>[2x]GSHMMPQLQFKDAFWCRDFTAHTGYEVLLQRLLDGRKMCKDMEELLRQRAQAEERYGKELVQIARKAGGQTEINSLRASFDSLKQQMENVGSSHIQLALTLREELRSLEEFRERQKEQRKKYEAVMDRVQKSKLSLYKKAMESKKTYEQKCRDADDAEQAFERISANGHQKQVEKSQNKARQCKDSATEAERVYRQSIAQLEKVRAEWEQEHRTTCEAFQLQEFDRLTILRNALWVHSNQLSMQCVKDDELYEEVRLTLEGCSIDADIDSFIQAKSTGTEPPAPVPYQNYYD;> GFANRFSKPKGPRNPPPTWNI

PSTPIP1 is an adaptor protein expressed in most immune cell lineages. It presents two structural domains in its sequence, an N-terminal Fer/CIP4 homology-Bin/Amphiphysin/Rvs (F-BAR) domain and a C-terminal SH3 domain, connected by a linker region. The F-BAR domain of PSTPIP1 binds to the PEST subfamily of protein tyrosine phosphatases (PTPs): PTPN12, also known as PTP-PEST, PTPN18, and the lymphoid phosphatase (LYP), encoded by the gene PTPN22. Positively charged residues on the concave surface of F-BAR domains interact with the polar heads of the phospholipids in the cellular membrane.

To visualize directly the PSTPIP1/LYP interaction we produced crystals of the F-BAR domain of PSTPIP1 in complex with a peptide of the CTH of LYP, residues 787–807. An additional continuous electron density, adjacent to PSTPIP1, was assigned to residues 793–806 of LYP. A single copy of LYP binds to the convex surface of the PSTPIP1 dimer at the rim of the dimerization interface formed by helices α4 of the two protomers. LYP buries ~ 625 Ǻ2 (2.1%) of the surface area of the PSTPIP1 dimer and establishes distinct contacts with each of the PSTPIP1 protomers; hereafter we refer to them as A and B. The LYP-binding site is characterized by three hydrophobic pockets aligned on the surface of PSTPIP1. P795 docks in a first pocket that is delimited by V243 and D246 of each protomer. D246 of protomer B also forms hydrogen bonds (H-bond) with the backbone amide groups of K796 and G797 of LYP. The side chain of the adjacent R799 makes ionic contacts with E250 and E257 of the protomer B; in addition, the main-chain amide and carbonyl of R799 make H-bonds with the side chain of N236 of protomer A. The C-terminal part of LYP (801–805) interacts with a deeper pocket formed between R228 and W232 of protomer A. P801 and P802 adopt a poly-proline II helix conformation; the ring of P801 contacts W232 in parallel. The first pocket of the LYP-binding site lies in the two-fold rotation axis that relates the two protomers of the PSTPIP1 dimer. Thus, only one molecule of LYP can bind to the PSTPIP1 dimer at any time. Finally, the conformation of the PSTPIP1 residues involved in LYP binding is very similar in the free and bound structures.> MNSNKDKIKVIKVFEAFAGIGSQFKALKNIARSKNWEIQHSGMVEWFVDAIVSYVAIHSKNFNPKIERLDRDILSISNDSKMPISEYGIKKINNTIKASYLNYAKKHFNNLFDIKKVNKDNFPKNIDIFTYSFPCQDLSVQGLQKGIDKELNTRSGLLWEIERILEEIKNSFSKEEMPKYLLMENVKNLLSHKNKKNYNTWLKQLEKFGYKSKTYLLNSKNFDNCQNRERVFCLSIRDDYLEKTGFKFKELEKVKNPPKK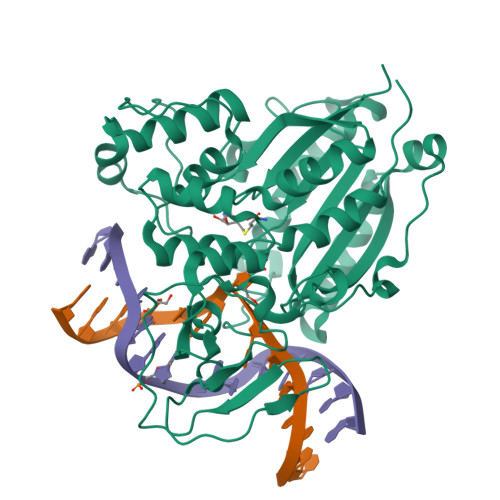IKDILVDSSNYKYLNLNKYETTTFRETKSNIISRPLKNYTTFNSENYVYNINGIGPTLTASGANSRIKIETQQGVRYLTPLECFKYMQFDVNDFKKVQSTNLISENKMIYIAGNSIPVKILEAIFNTLEFVNNEELEHHHHHH> AMSDLELRQCLPCGPGGKGRCFGPSICCGDELGCFVGTAEALRCQEENYLPSPCQSGQKPCGSGGRCAAAGICCNDESCVTEPE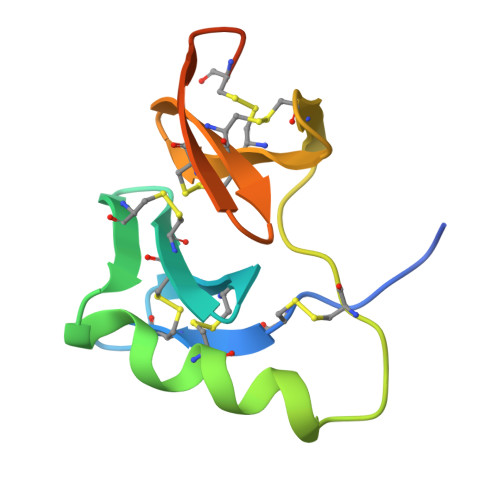CREGVGFPRRV> MAESKSITFELNESVLTAQVGRLDEMAMVVERRFSELKMTIEDVGNADPGSKISESLGGLQSGLGTIS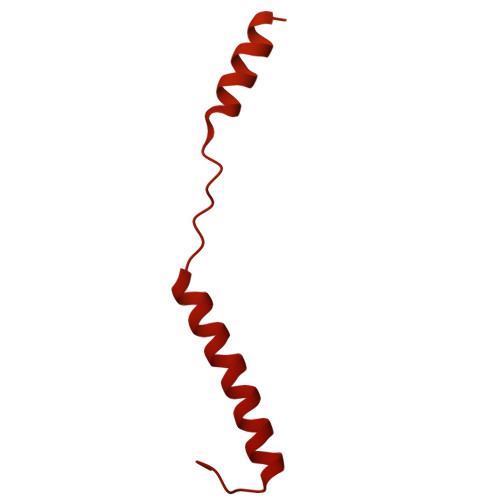SAFGQLGSSSEAITSGFGTAVGSVGGITDAFKNLGSSVQNGTLFSSLATGIGGMSTMLGGVSGGVQGITNLASGFMELKNHLGGLMSSIGGVGGIMGKLTSPMGLVIIGIVALVAAFTYLMTTNESFRNTVMSVVTQVAQLFGQLVASLMPIIMQIVTAVMQIGAALMPMVMQFISFFAQLLAQLMPFINMLISMLMPVIMQIVQVVMSLVSALLPSIMTVIQGIMSVIQFLIPIIMQIATVVVQIVVTIISYISKIMPIVMTIIGVIVSIITTIISYVVIIATTIASVIGKIISFIASVITAVIGIVQPIIAFITNIFTTIVTIIGAAFQMVFTVASKIWNSIMSTISGIIDGIKAVITGISTTVSSVFNGVKRIITGVFDGIKSAWGGLTDFVGNIFDGVSSAIQTVVDNVKGFVNVVIRGINGAIGLINKIPGVEIGKIPQLISGTTNFQGGFARMNEGGRGEMVVLPSGSQVIPHDATMKYARESARGNKSMLYTSQGADLARVENLLERLLQKNPVIKMDDKVVAEVVSRNQANSFDQYNYTMGGAAYS>[3x]GSRAQSSPAAPASLSAPEPASQARVLSSSETPARTLPFTTGLIYDSVMLKHQCSCGDNSRHPEHAGRIQSIWSRLQERGLRSQCECLRGRKASLEELQSVHSERHVLLYGTNPLSRLKLDNGKLAGLLAQRMFVMLPCGGVGVDTDTIWNELHSSNAARWAAGSVTDLAFKVASRELKNGFA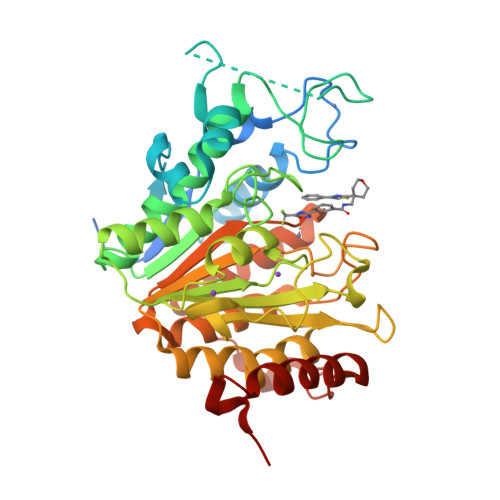VVRPPGHHADHSTAMGFCFFNSVAIACRQLQQQSKASKILIVDWDVHHGNGTQQTFYQDPSVLYISLHRHDDGNFFPGSGAVDEVGAGSGEGFNVNVAWAGGLDPPMGDPEYLAAFRIVVMPIAREFSPDLVLVSAGFDAAEGHPAPLGGYHVSAKCFGYMTQQLMNLAGGAVVLALEGGHDLTAICDASEACVAALLGNRVDPLSEEGWKQKPNLNAIRSLEAVIRVHSKYWGCMQRLAS(1S,2R)-2-[(S)-amino(carboxy)methyl]cyclobutanecarboxylic 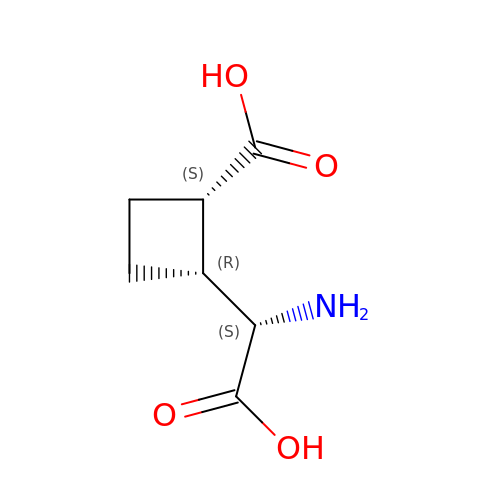acid | C7 H11 N O4 | SRAFHGOPGVYULO-WISUUJSJSA-N>MDVASLPGKLADCSSKSPEECEIFLVEGDSAGGSTKSGRDSRTQAILPLRGKILNVEKARLDRILNNNEIRQMITAFGTGIGGDFDLAKARYHKIVIMTDADVDGAHIRTLLLTFFYRFMRPLIEAGYVYIAQPPLYKLTQGKQKYYVYNDRELDKLKSELNPTPKWSIARYKGLGEMNADQLWETTMNPEHRALLQVKLEDAIEADQTFEMLMGDVVENRRQFIEDNAVYANLDFAELPQSRINERNITSEMRESFLDYAMSVIVARALPDVRDGLKPVHRRILYGLNEQGMTPDKSYKKSARIVGDVMGKYHPHGDSSIYEAMVRMAQDFSYRYPLVDGQGNFGSMDGDGAAAMRFTEARMTKITLELLRDINKDTIDFIDNYDGNEREPSVLPARFPNLLANGASGIAVGMATNIPPHNLTELINGVLSLSKNPDISIAELMEDIEGPDFPTAGLILGKSGIRRAYETGRGSIQMRSRAVIEERGGGRQRIVVTEIPFQVNKARMIEKIAELVRDKKIDGITDLRDETSLRTGVRVVIDVRKDANASVILNNLYKQTPLQTSF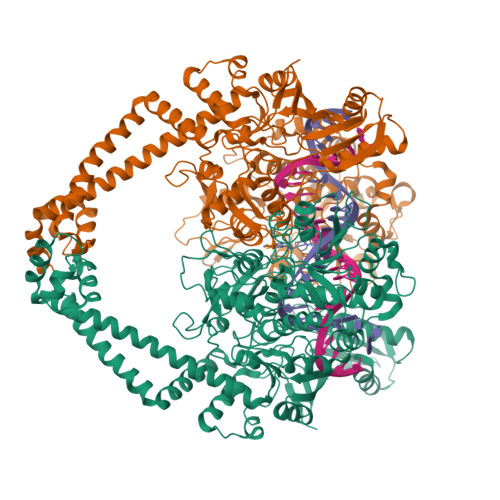GVNMIALVNGRPKLINLKEALVHYLEHQKTVVRRRTQYNLRKAKDRAHILEGLRIALDHIDEIISTIRESDTDKVAMESLQQRFKLSEKQAQAILDMRLRRLTGLERDKIEAEYNELLNYISELETILADEEVLLQLVRDELTEIRDRFGDDRRTEIQLG[4x]> GLVPRGSHMMEILRGSPALSAFRINKLLARFQAANLQVHNIYAEYVHFADLNAPLNDSEQAQLTRLLQYGPALSSHTPAGKLLLVTPRPGTISPWSSKATDIAHNCGLQQVDRLERGVAYYIEASTLTAEQWRQVAAELHDRMMETVFSSLTDAEKLFIHHQPAPVSSVDLLGEGRQALIDANLRLGLALAEDEIDYLQEAFTKLGRNPNDIELYMFAQANSEHCRHKIFNADWIIDGKPQPKSLFKMIKNTFETTPDYVLSAYKDNAAVMEGSAVGRYFADHNTGRYDFHQEPAHILMKVETHNHPTAISPWPGAATGSGGEIRDEGATGRGAKPKAGLVGFSVSNLRIPGFEQPW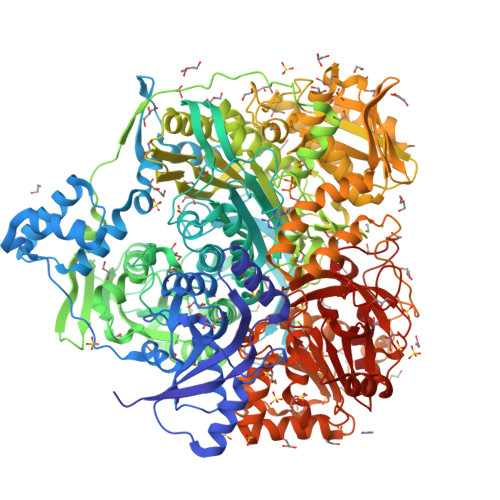EEDFGKPERIVTALDIMTEGPLGGAAFNNEFGRPALTGYFRTYEEKVNSHNGEELRGYHKPIMLAGGIGNIRADHVQKGEIVVGAKLIVLGGPAMNIGLGGGSSMASGQSDADLDFASVQRDNPEMERRCQEVIDRCWQLGDANPILFIHDVGAGGLSNAMPELVSDGGRGGKFELRDILSDEPGMSPLEIWCNESQERYVLAVAADQLPLFDELCKRERAPYAVIGDATEEQHLSLHDNHFDNQPIDLPLDVLLGKTPKMTRDVQTLKAKGDALNRADITIADAVKRVLHLPTVAEKTFLVTIGDRTVTGMVARDQMVGPWQVPVADCAVTTASLDSYYGEAMSIGERAPVALLDFAASARLAVGEALTNIAATQIGDIKRIKLSANWMAAAGHPGEDAGLYDAVKAVGEELCPQLGLTIPVGKDSMSMKTRWQEGNEQREMTSPLSLVISAFARVEDVRHTLTPQLSTEDNALLLIDLGKGHNALGATALAQVYRQLGDKPADVRDVAQLKGFYDAMQALVAARKLLAWHDRSDGGLLVTLAEMAFAGHCGVQVDIAALGDDHLAALFNEELGGVIQVRAEDRDAVEALLAQYGLADCVHYLGQALAGDRFVITANDQTVFSESRTTLRVWWAETTWQMQRLRDNPQCADQEHEAKANDTDPGLNVKLSFDINEDIAAPYIATGARPKVAVLREQGVNSHVEMAAAFHRAGFDAIDVHMSDLLGGRIGLGNFHALVACGGFSYGDVLGAGEGWAKSILFNHRVRDEFETFFHRPQTLALGVCNGCQMMSNLRELIPGSELWPRFVRNHSDRFEARFSLVEVTQSPSLLLQGMVGSQMPIAVSHGEGRVEVRDDAHLAALESKGLVALRYVDNFGKVTETYPANPNGSPNGITAVTTENGRVTIMMPHPERVFRTVANSWHPENWGEDSPWMRIFRNARKQLG octyl 3-deoxy-2-O-(6-deoxy-alpha-L-galactopyranosyl)-beta-D-xylo-hexopyranoside | 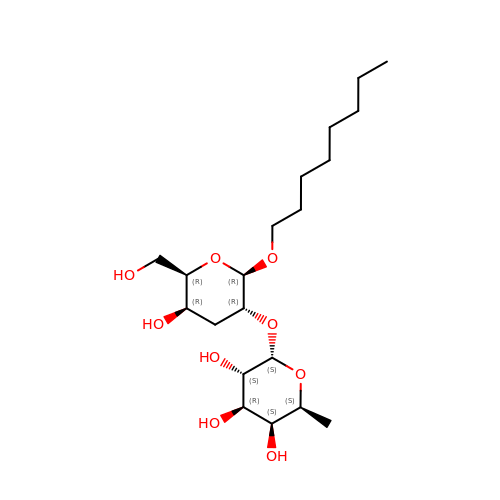C20 H38 O9 | FBVFDKBCZLMLQT-PPCMOIRNSA-N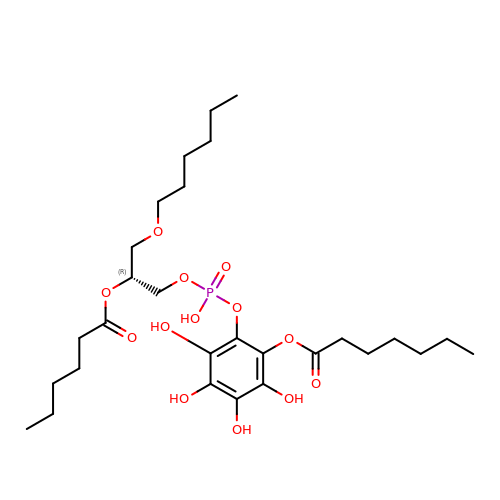[2-[[(2~{R})-2-hexanoyloxy-3-[(~{E})-hex-3-enoxy]propoxy]-oxidanyl-phosphoryl]oxy-3,4,5,6-tetrakis(oxidanyl)phenyl] (2~{E},4~{E})-hepta-2,4-dienoate | C28 H47 O13 P | JZBYPPGRAPDSFI-HXUWFJFHSA-N>[2x]MRRSVYLDNTIEFLRGRVYLGAYDYTPEDTDELVFFTVEDAIFYNSFHLDFGPMNIGHLYRFAVIFHEILNDPENANKAVVFYSSASTRQRANAACMLCCYMILVQAWTPHQVLQP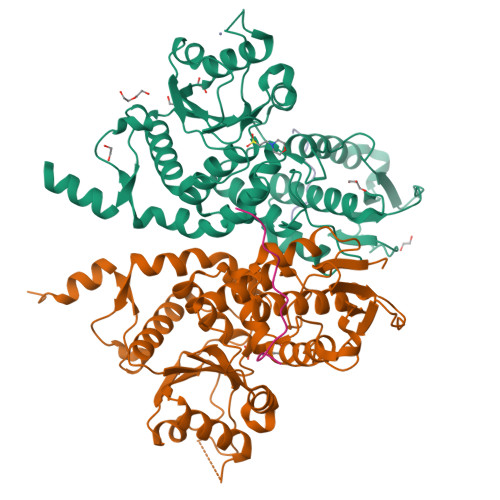LAQVDPPFMPFRDAGYSNADFEITIQDVVYGVWRAKEKGLIDLHSFNLESYEKYEHVEFGDFNVLTPDFIAFASPQEDHPKGYLATKSSHLNQPFKSVLNFFANNNVQLVVRLNSHLYNKKHFEDIGIQHLDLIFEDGTCPDLSIVKNFVGAAETIIKRGGKIAVHCKAGLGRTGCLIGAHLIYTYGFTANECIGFLRFIRPGMVVGPQQHWLYLHQNDFREWKYTTRISLKPSEAIGGLYPLISLEEYRLQKKKLKD;> FTDVPALNYPATPPPH;> AFTDVPALNYPATPPPH1-hydroxy-2-methyl-3-[(2E,6E)-3,7,11-trimethyldodeca-2,6,10-trien-1-yl]quinolin-4(1H)-one | C25 H33 N O2 | 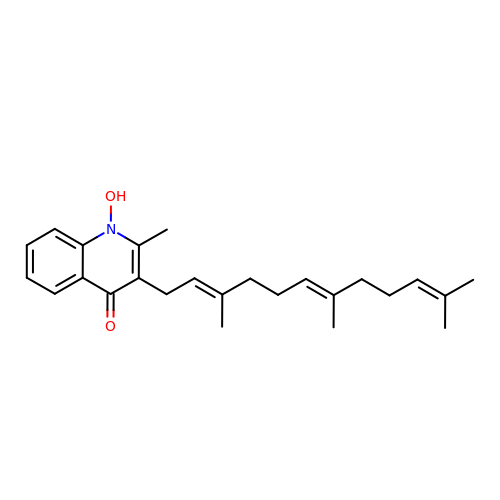FIHXCHBEHLCXEG-YEFHWUCQSA-N> MSNLNVERVLSVHHWNDTLFSFKTTRNPSLRFENGQFVMIGLEVDGRPLMRAYSIASPNYEEHLEFFSIKVQNGPLT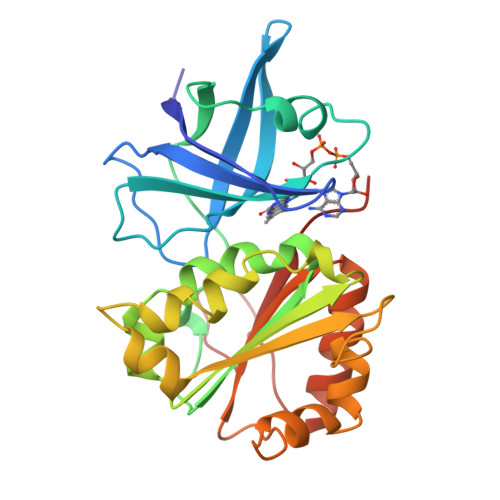SRLQHLKEGDELMVSRKPTGTLVTSDLLPGKHLYMLSTGTGLAPFMSLIQDPEVYERFEKVVLIHGVRQVNELAYQQFITEHLPQSEYFGEAVKEKLIYYPTVTRESFHNQGRLTDLMRSGKLFEDIGLPPINPQDDRAMICGSPSMLDESCEVLDGFGLKISPRMGEPGDYLIERAFVEK> KPLQNWEQASPGENAHSSLGLSGAGEEGVFDLQMFLENMKVDFLRSLNLSGIPSQDKTRAEPPQYMIDLYNRYTTDKSSTPASNIVRSFSVEDAISTAATEDFPFQKHILIFNISIPRHEQITRAELRLYVSCQNDVDSTHGLEGSMVVYDVLEDSETWDQATGTKTFLVSQDIRDEGWETLEVSSAVKRWVRADSTTNKNKLEVTVQSHRESCDTLDISVPPGSKNLPF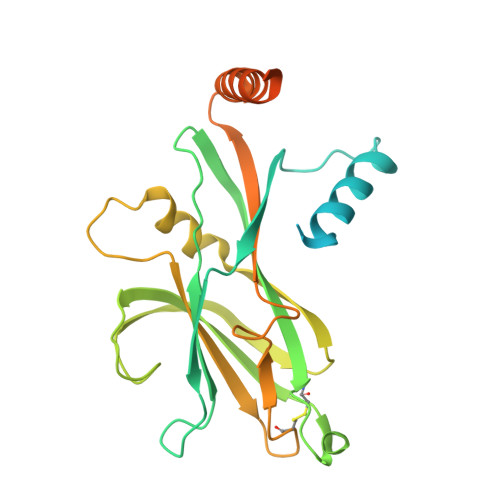FVVFSNDRSNGTKETRLELKEMIGHEQETMLVKTAKNAYQVAGESQEEEGLDGYTAVGPLLARRKR>[4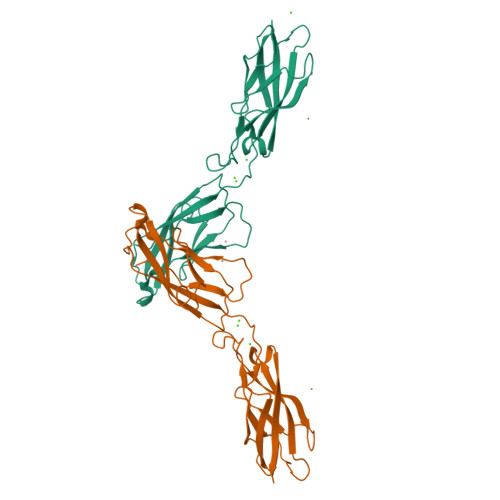x]EWVMPPIFVPENGKGPFPQRLNQLKSNKDRGTKIFYSITGPGADSPPEGVFTIEKESGWLLLHMPLDREKIVKYELYGHAVSENGASVEEPMNISIIVTDQNDNKPKFTQDTFRGSVLEGVMPGTSVMQVTATDEDDAVNTYNGVVAYSIHSQEPKEPHDLMFTIHKSTGTISVISSGLDREKVPEYRLTVQATDMDGEGSTTTAEAVVQILD>[2x]MSFNESASIPTGLTYDDVLIIPQHSRVTSRKEVNTTTRLSRNVKLSIPIVASNMDTVCEQRMAVAMAREGGIGILHRFCSIEEQCAMLREVKRAQSFLIESPRIILPHETAREAWEGLNWKGRVGGVGCLLVVNCKNERKLLGIITRHDLKLADESTTVESLMTPVDKMVVSTNTSISLEEVTHLMRKGRTANVPIVGQNGQLLYLVTLSDVVKLRKNKQASLDSRGRLLVGAAVGVKKDDMNRAIRLVEAGADVLVVDIAHGHSDLCINMVKRLKGDPRTASVDIIAGNIASAEAAEALIDAGADGLKIGVGPGSIAITRLVAGAGVPQLSAVLACTRVARRRGVPCIADGGLRTSGDISKAIGAGADTVMLGNMLAGTDEAPGRVLVKDGQKVKIIRGMAGFGANLSKAERERTQDEDVFSSLVPEGVEGSVACKGPVGPIVRQLVGGLRSGMSYSGAKSIEEMQRRTRFVRMTGAGLRESGSHGVAKLKLAAALEHHHHHH

Here, we demonstrate the determination of the crystal structures of T. brucei GMPR; a protein that, unlike the GMPRs of host animals, possesses a CBS domain. We further show that TbGMPR activity is regulated by purine nucleotide binding to an allosteric regulatory site formed at the cleft between the catalytic and CBS domains of the enzyme. Our kinetic and structural analyses clearly demonstrate that the CBS domain has a pivotal role in the allosteric regulation of the activity and structure of TbGMPR, facilitating the transitions among three conformations: a tetramer, and octamers with relaxed and twisted conformations. A combination of X-ray crystallography and size-exclusion chromatography small-angle X-ray scattering (SEC-SAXS) analysis clearly revealed that TbGMPR can exist as a tetramer or an octamer depending on the nucleotide species that is bound to the CBS domain.

To obtain direct evidence for the allosteric binding of purine nucleotides to the CBS domain of TbGMPR, we attempted crystallization, with or without purine nucleotides, of the inactive mutant TbGMPR C318A, in which the catalytic residue Cys3186 was replaced by an alanine. We obtained the crystal without ligand (C318A apo) and successfully determined the structure, at 2.80-Å resolution, of a GMPR harboring a CBS domain. A monomer of C318A apo comprised two domains: the catalytic domain (Ser2–Phe97 and Arg226–Gly484) and the CBS domain (Leu98–Ser225). The former displayed a typical TIM-barrel fold with accessory α-helices and antiparallel β-sheets, whereas the latter had a tandem repeat of α–β–β–α folds characteristic to all CBS domains known to date. The interactions between the adjacent subunits in the tetramer involved a large number of hydrogen bonds and hydrophobic interactions, whereas the formation of the octamer was stabilized by a hydrogen bond and 14 C–C contacts between the CBS domains of subunit A in tetramer 1 and subunit A′ in tetramer 2, and equivalent interactions between subunit B and B′, C and C′, and D and D′. However, no interaction was observed between the catalytic domains, indicating that the CBS domain is essential for the formation of the TbGMPR octamer. Thus, it appears that GMP induces the transformation of TbGMPR from a “relaxed” (C318A apo) to a “twisted” form (C318A/GMP). However, the relative orientation of these domains was obviously different between C318A/GMP and C318A apo: the CBS domain is rotated ~40° between these two structures, a change that may be induced by an interaction between the base moiety of GMP and Arg93. Two of the three conformations were the crystal structures of C318A apo and C318A/GMP that represent the relaxed and the twisted octamers, respectively; the third conformation was a tetramer structure generated by dividing the C318A/GMP octamer in half.> VPIRQLHYRLRDEQQKSLVLSDPYELKALHLNGQNINQQVIFSMSFVQGEPSNDKIPVALGLKGKNLYLSCVMKDGTPTLQLESVDPKQYPKKKMEKRFVFNKIEVKSKVEFESA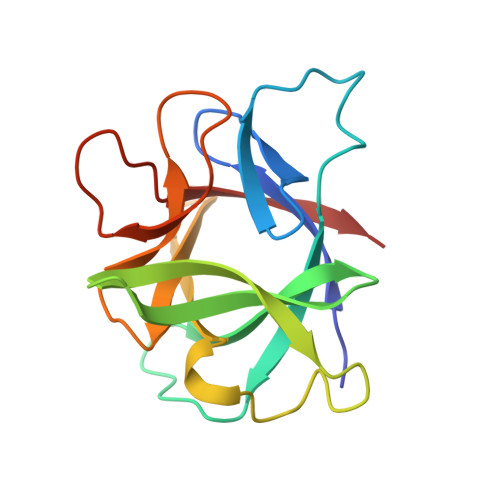EFPNWYISTSQAEHKPVFLGNNSGQDIIDFTMESVSS>[4x]GSHMASGEGPALYEDPPDQKTSPSGKPATLKICSWNVDGLRAWIKKKGLDWVKEEAPDILCLQETKCSENKLPAELQELPGLSHQYWSAPSDKEGYSGVGLLSRQCPLKVSYGIGDEEHDQEGRVIVAEFDSFVLVTAYVPNAGRGLVRLEYRQRWDEAFRKFLKGLASRKPLVLCGDLNVAHEEIDLRNPKGNKKNAGFTPQERQGFGELLQAVPLADSFRHLYPNTPYAYTFWTYMMNARSKNVGWRLDYFLLSHSLLPALCDSKIRSKALGSDHCPITLYLAL

Mammalian AP endonuclease 1 (APE1) initiates repair of abasic (apurinic/apyrimidinic) sites and other toxic and mutagenic DNA lesions and performs critical roles in base excision repair (BER) and single strand break repair (SSBR). APE1 hydrolytically cleaves phosphodiester bonds at abasic sites, which arise through spontaneous rupture of the N-glycosyl bond (depurination) or by the activity of DNA glycosylases, which initiate BER. APE1 is the major mammalian enzyme for repair of abasic sites, which impair DNA replication and other processes, causing DNA strand breaks and cross links. In addition to its AP endonuclease activity, the exonuclease activity of APE1 processes BER intermediates generated by bifunctional DNA glycosylases and removes 3´-blocking groups arising at strand breaks.

We also sought to obtain a crystal structure of APE1 in complex with one of the indole compounds and found success with 5-nitroindole-2-carboxylic acid. The crystals used to determine the structure of APE1 in complex with 3 were generated by soaking preformed crystals of apo APE1 in a solution of mother liquor with 5% DMSO and 100 mM compound 3. While this concentration of 3 is two orders of magnitude above that observed to form aggregates, our result indicates that some fraction of the compound, perhaps a small fraction, is populated in the monomeric form under the crystallization conditions. Compound 3 features strong electron density, defining its pose and binding interactions with the enzyme. Additional evidence for binding of compound 3 to this remote pocket is provided by the Fo-Fc map calculated using a model that does not include the compound The 5-nitro of 3 accepts hydrogen bonds from S135 and R136 and the backbone N of Q137, and the 2-carboxyl of 3 is contacted by the hydroxyl and the backbone N of S164. The pocket features many hydrophobic residues, including L62, I64, I91, F162, and F165. Together, these nine residues are among the 11 that exhibit the largest NMR CSPs (Δδ ≥ 0.03 ppm) induced by 3, demonstrating excellent agreement between the crystallographic and NMR results. Regarding APE1 conformational changes caused by the binding of compound 3, superposition of our two new structures for apo APE1, free and in complex with compound 3, reveals that binding of 3 induces minor changes in overall structure with some significant changes in the remote binding site for residues including L62, D90, R136, Q137, F162, S164, F165, and L318. Remarkably, our results also show that the indole compounds bind at a pocket of APE1 that is distal from its active site, with specific interactions defined in a crystal structure of APE1 in complex with compound 3. However, the activity assays show that these compounds inhibit APE1 only under conditions that permit compound aggregation and not under conditions that disrupt it (with detergent).> SSADRLFPPQWICCDIRYLDVSILGKFAVVMADPPWDIHMELPYGTLTDDEMRRLNIPVLQDDGFLFLWVTGRAMELGRECLNLWGYERVDEIIWVKTNQLQRIIRTGRTGHWLNHGKEHCLVGVKGNPQGFNQGLDCDVIVAEVRSTSHKPDEIYGMIERLS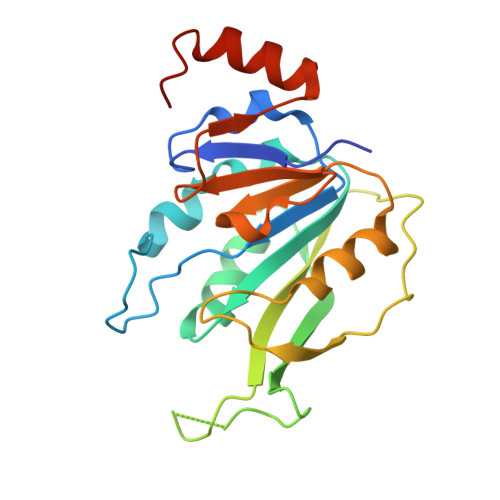PGTRKIELFGRPHNVQPNWITLGNQLDGIHLLDPDVVARFKQRYPDGIISKPKNL> MGHNHRHKHHHHHHHHENLYFQGPGSSPSLEQDDGDEETSVVIVGKISFCPKDVLGHGAEGTIVYRGMFDNRDVAVKRILPECF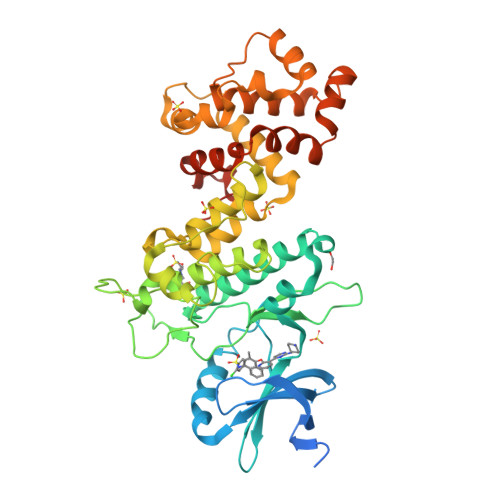SFADREVQLLRESDEHPNVIRYFCTEKDRQFQYIAIELCAATLQEYVEQKDFAHLGLEPITLLQQTTSGLAHLHSLNIVHRDLKPHNILISMPNAHGKIKAMISDFGLCKKLAVGRHSFSRRSGVPGTEGWIAPEMLSEDCKENPTYTVDIFSAGCVFYYVISEGSHPFGKSLQRQANILLGACSLDCLHPEKHEDVIARELIEKMIAMDPQKRPSAKHVLKHPFFWSLEKQLQFFQDVSDRIEKESLDGPIVKQLERGGRAVVKMDWRENITVPLQTDLRKFRTYKGGSVRDLLRAMRNKKHHYRELPAEVRETLGTLPDDFVCYFTSRFPHLLAHTYRAMELCSHERLFQPYYFHEPPEPQPPVTPDAL> ATRRYYLGAVELSWDYMQSDLGELPVDARFPPRVPKSFPFNTSVVYKKTLFVEFTDHLFNIAKPRPPWMGLLGP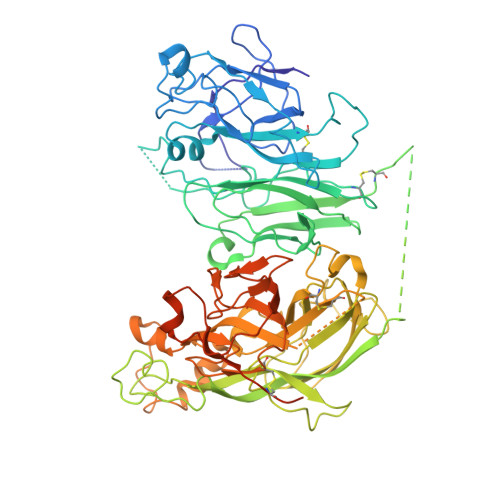TIQAEVYDTVVITLKNMASHPVSLHAVGVSYWKASEGAEYDDQTSQREKEDDKVFPGGSHTYVWQVLKENGPMASDPLCLTYSYLSHVDLVKDLNSGLIGALLVCREGSLAKEKTQTLHKFILLFAVFDEGKSWHSETKNSLMQDRDAASARAWPKMHTVNGYVNRSLPGLIGCHRKSVYWHVIGMGTTPEVHSIFLEGHTFLVRNHRQASLEISPITFLTAQTLLMDLGQFLLFCHISSHQHDGMEAYVKVDSCPEEPQLRMKNNEEAEDYDDDLTDSEMDVVRFDDDNSPSFIQIRSVAKKHPKTWVHYIAAEEEDWDYAPLVLAPDDRSYKSQYLNNGPQRIGRKYKKVRFMAYTDETFKTREAIQHESGILGPLLYGEVGDTLLIIFKNQASRPYNIYPHGITDVRPLYSRRLPKGVKHLKDFPILPGEIFKYKWTVTVEDGPTKSDPRCLTRYYSSFVNMERDLASGLIGPLLICYKESVDQRGNQIMSDKRNVILFSVFDENRSWYLTENIQRFLPNPAGVQLEDPEFQASNIMHSINGYVFDSLQLSVCLHEVAYWYILSIGAQTDFLSVFFSGYTFKHKMVYEDTLTLFPFSGETVFMSMENPGLWILGCHNSDFRNRGMTALLKVSSCDKNTGDYYEDSYEDISAYLLSKNNAIEPRSFSQNSRHPSQNPPVLKRHQ3,6-dimethyl-~{N}-[4-(trifluoromethyl)phenyl]-[1,2]oxazolo[5,4-d]pyrimidin-4-amine 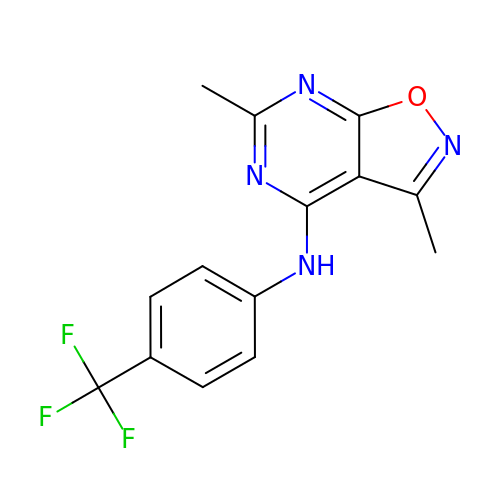| C14 H11 F3 N4 O | DICIXXZXANPVKT-UHFFFAOYSA-N N-{(2S)-3-[(R)-(4-bromophenyl)(hydroxy)phosphoryl]-2-[(3-phenyl-1,2-oxazol-5-yl)methyl]propanoyl}-L-alanyl-L-alaninamide | C25 H28 Br N4 O6 P | 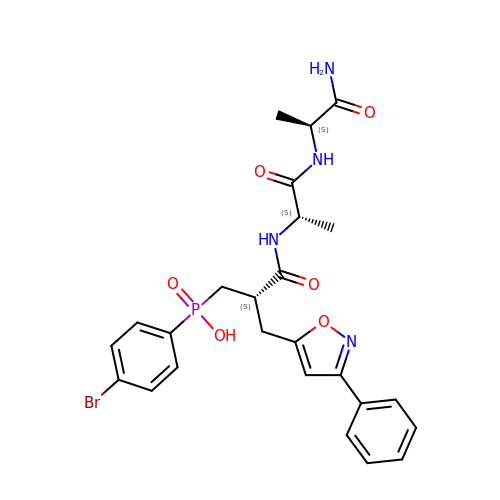HXHLWPVBBLIGJV-XYJFISCASA-N> MFKDFFNRTKKKKYLTVQDSKNNDVPAGIMTKCPKCKKIMYTKELAENLNVCFNCDHHIALTAYKRIEAISDEGSFTEFDKGMTSANPLDFPSYLEKIEKDQQKTGLKEAVVTGTAQLDGMKFGVAVMDSRFRMGSMGSVIGEKICRIIDYCTENRLPFILFSASGGARMQEGIISLMQMGKTSVSLKRHSDAGLLYI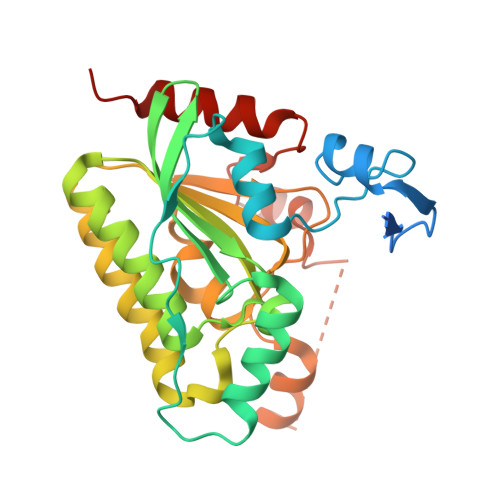SYLTHPTTGGVSASFASVGDINLSEPKALIGFAGRRVIEQTINEKLPDDFQTAEFLLEHGQLDKVVHRNDMRQTLSEILKIHQEVTK> DHPFTEIKSGFLERRSKFLKSYSKGYYVLTPNFLHEFKTADRKKDLVPVMSLALSECTVTEHSRKNSTSSPNSTGSDAKFVLHAKQNGIIRRGHN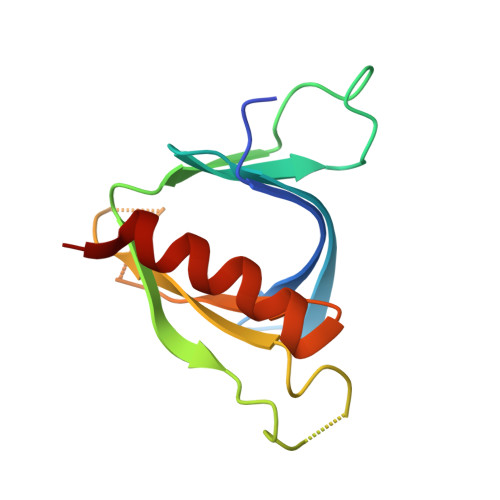YVFKADSYESMMSWFDNLKILTSTS> ALSAYSLRSLIVTYNSRNRSSMNATIENLKNALRWTSPSESSSPSSAPSSAPSSAPSSSWSPPWPVPRRVGRRQWRVTYLKSPFKYKYALRHYVFEDHRYAFAFYDVNSVQEVVSAALGAMAGETCCSCRFSWRFAGRPPVSLPTPPRLVPSSRAASLLSSRSSSEDGEVSREPVEGGEKTSGVKKAPHLAT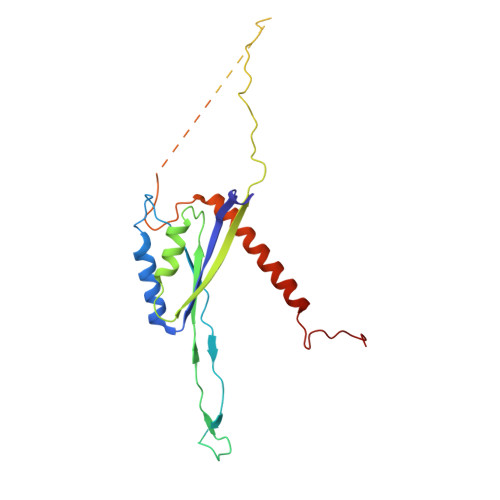VLRGHCPTDKEFIRRALEEEQAVERIRKKLDKKQLQWFPGKTPWAP>GQEPENQTLETILNRKSVRKYKDRPVEKEKIDKLIRAGMAAPSSRDRRPWEFIIVTDRKALDTMAEGLPFARMLKETRQAIVVCGDTIKSSNAWFLDCSAASQNLLLAAESMGLGAVWTAVYPYPDRIEIVRKELRLPDHIMPLNVIPVGYPMQKETPKNKYNVQQIH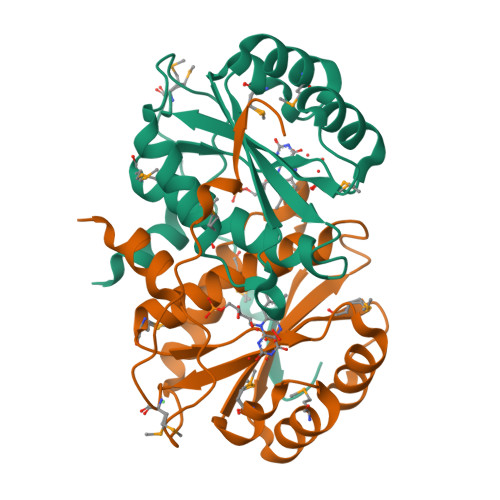HNGW[2x]> EFPEITEEMEKEIKNVFRNGNQDEVLSEAFRLTITRKDIQTLNHLNWLNDEIINFYMNMLMERSKEKGLPSVHAFNTFFFTKLKTAGYQAVKRWTKKVDVFSVDILLVPIHLGVHWCLAVVDFRKKNITYYDSMGGIN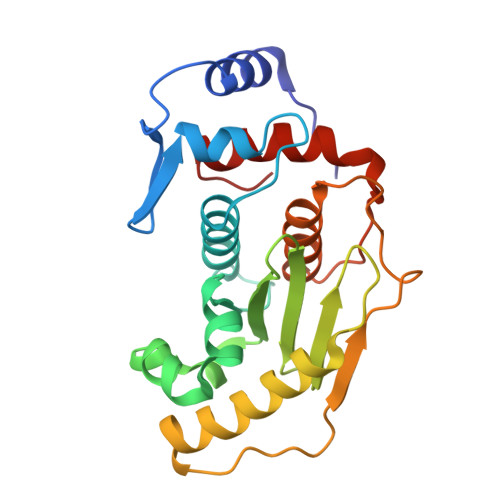NEACRILLQYLKQESIDKKRKEFDTNGWQLFSKKSQEIPQQMNGSDAGMFACKYADCITKDRPINFTQQHMPYFRKRMVWEILHRKLL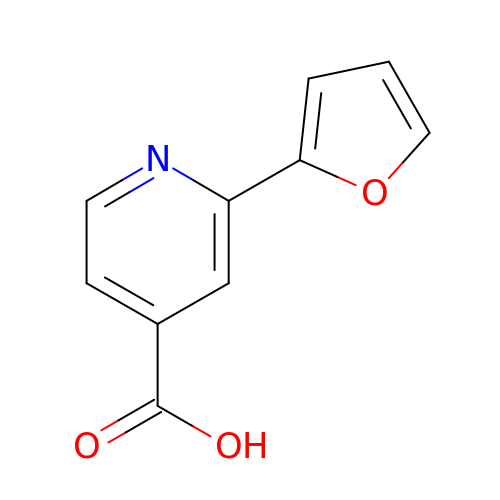2-(furan-2-yl)pyridine-4-carboxylic acid | C10 H7 N O3 | RDJBDQGUVODXPZ-UHFFFAOYSA-N>[2x]MSNIQNMSLEDIMGERFGRYSKYIIQDRALPDIRDGLKPVQRRILYSMNKDSNTFDKSYRKSAKSVGNIMGNFHPHGDSSIYDAMVRMSQNWKNREILVEMHGNNGSMDGDPPAAMRYTEARLSEIAGYLLQDIEKKTVPFAWNFDDTEKEPTVLPAAFPNLLVNGSTGISAGYATDIPPHNLAEVIDAAVYMIDHPTAKIDKLMEFLPGPDFPTGAIIQGRDEIKKAYETGKGRVVVRSKTEIEKLKGGKEQIVITEIPYEINKANLVKKIDDVRVNNKVAGIAEVRDESDRDGLRIAIELKKDANTELVLN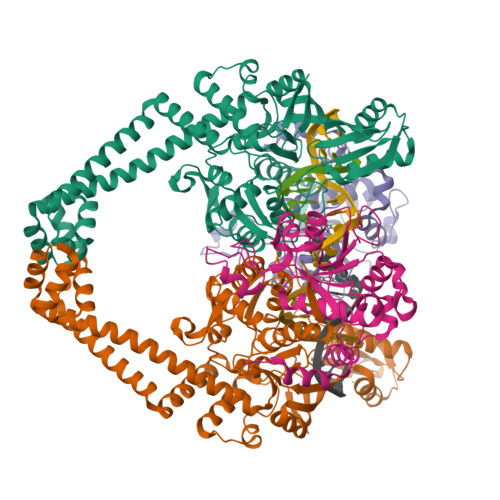YLFKYTDLQINYNFNMVAIDNFTPRQVGIVPILSSYIAHRREVILARSRFDKEKAEKRLHIVEGLIRVISILDEVIALIRASENKADAKENLKVSYDFTEEQAEAIVTLQLYRLTNTDVVVLQEEEAELREKIAMLAAIIGDERTMYNLMKKELREVKKKFATPRLSSLEDTAKALEHHHHHH;>MGHHHHHHHHHHSSGHIDDDDKHMKNKKDKGLLSGKLTPAQSKNPAKNELYLVEGDSAGGSAKQGRDRKFQAILPLRGKVINTAKAKMADILKNEEINTMIYTIGAGVGADFSIEDANYDKIIIMTDADTDGAHIQTLLLTFFYRYMRPLVEAGHVYIALPPLYKMSKGKGKKEEVAYAWTDGELEELRKQFGKGATLQRYKGLGEMNADQLWETTMNPETRTLIRVTIEDLARAERRVNVLMGDKVEPRRKWIEDNVKFTLEEATVF[2x]>GSMTQIHQINDIDVHRITSGQVITDLTTAVKELVDNSIDANANQIEIIFKDYGLESIECSDNGDGIDPSNYEFLALKHYTSKIAKFQDVAKVQTLGFRGEALSSLCGIAKLSVITTTSPPKADKLEYDMVGHITSKTTTSRNKGTTVLVSQLFHNLPVRQKEFSKTFKRQFTKCLTVIQGYAIINAAIKFSVWNITPKGKKNLILSTMRNSSMRKNISSVFGAGGMRGLEEVDLVLDLNPFKNRMLGKYTDDPDFLDLDYKIRVKGYISQNSFGCGRNSKDRQFIYVNKRPVEYSTLLKCCNEVYKTFNNVQFPAVFLNLELP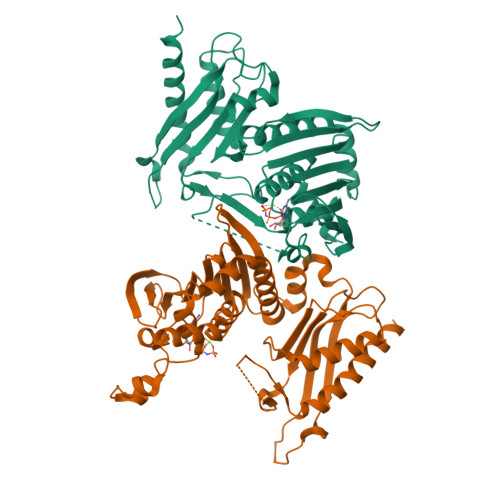MSLIDVNVTPDKRVILLHNERAVIDIFKTTLSDYYNRQELALPK[2x]> GSHMASMATGSEASKAAEAVVDWHKHDSKRMLHAVYRVGDLDRTIKYYTECFGMKLLRKRDVPDEKYTNAFLGFGPENTNFAVELTYNYGVDKYDIGTGFGHFAIANDDVYKLAENIKSKGGKITREPGPVKGGSTVIAFAQDPDGYMFELIQRADTPEPLCQVMLRVGDLERSIKFYEKALGMKLLRKKDVPDYKYTIAMLGYADEDKTTVLELTYNYGVTEYSKGNAYAQVAIGTNDVYKSAEA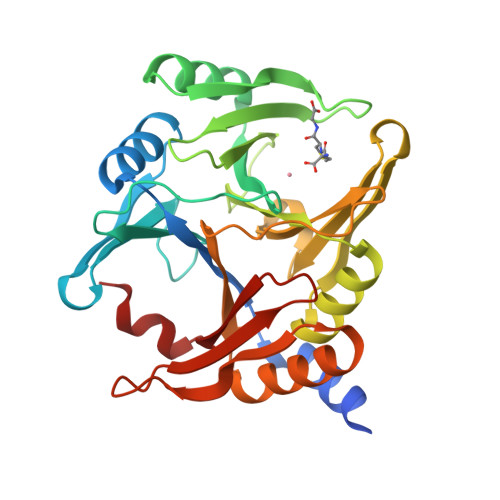VDLATKELGGKILRQPGPLPGINTKIASFVDPDGWKVELVDNTDFLKELH> MELENIVANTVLLKAREGGGGKRKGKSKKWKEILKFPHISQCEDLRRTIDRDYCSLCDKQPIGRLLFRQFCETRPGLECYIQFLDSVAEYEVTPDEKLGEKGKEIMTKYLTPKSPVFIAQVGQDLVSQTEEKLLQKPCKELFSACAQSVHEYLRGEPFHEYLDSMFFDRFLQWKWLERQPVTKNTFRQYRVLGKGGFGEVCACQVRATGKMYACKRLEKKRIKKRKGESMALNEKQILEKVNSQFVVNLAYAYETKDALCLVLTIMNGGDLKFHIYNMGNPGFEEERALFYAAEILCGLEDLHRENTVYRNLKPENILLDDYGHIRISDLGLAVKIPEGDLIRGRVGTVGYMAPEVLNNQRYGLSPDYWGLGCLIYEMIEGQSPFRGRKEKVKREEVDRRVLETEEVYSHKFSEEAKSICKMLLTKDAKQRLGCQEEGAAEVKR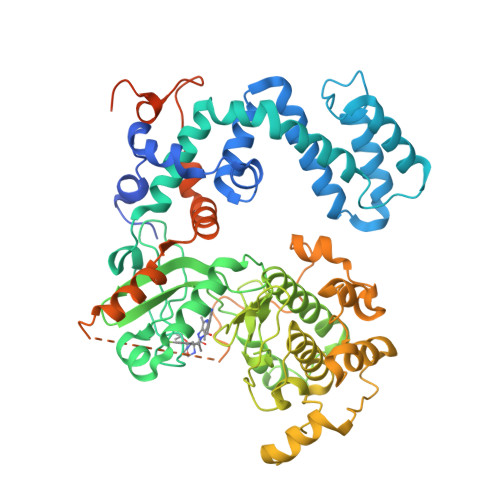HPFFRNMNFKRLEAGMLDPPFVPDPRAVYCKDVLDIEQFSTVKGVNLDHTDDDFYSKFSTGSVSIPWQNEMIETECFKELNVFGPNGTLPPDLNRNHPPEPPKKGLLQRLFKRQHQNNSKSSPSSKTSFNHHINSNHVSSNSTGSSVDHHHHHH> MAPVPEPEVVATPPADAGRGLIRVDSREIRHYSGTRKEPDYLVSRDNGKTWEMKAAPAGYPPNYGGIPKESPAIVRNPLTREFIRVQPIGGFVFLSRGGLDGKWLAVTNDGKLEEDWKDPEKRKNLKKLGGIMRTPVFVNKGRRVIVPFHNMGGGTKFHISDDGGLTWHVSRNGVTSPRHEARPPHQGVRWFNNAVEA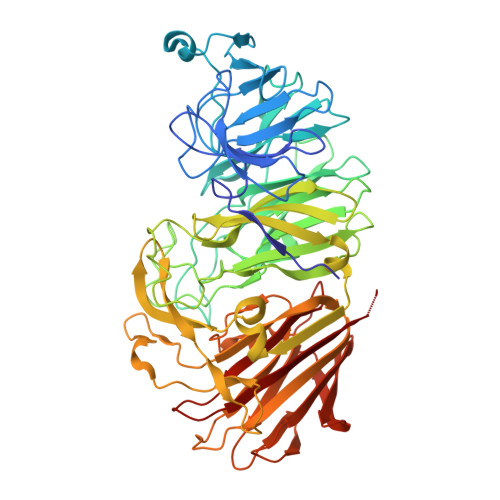TVLEMKDGTLWALARTSQDQAWQAFSKDYGETWSKPEPSRFFGTLTMNTLGRLDDGTIVSLWTNTMALPENATAGNGTWEDVFTNRDSHHIAMSGDEGKTWYGFREIILDEHRNHPGYATLDGPEDRGKHQSEMVQLDKNRILISLGQHKNHRRLVIVDRRWVGAKTRATQTGKDLDSQWTIHTYIPQKKGHCSYNRKPSAELVQDPSGGTKKVLQIKRLDDPELVNEKSNVDYRNGGATWNFPNGTTGLVKFRFRVVDGEQADDSGLQVSLTDRLFNACDSTTKDYALFTFPIRLKPAPHLLLGMKKVPFTPGAWHEISLLWQGGQAVVSLDGKKAGTLKMANKSPNGASYIHFISTGSQPDAGILLDTVNARVKAAAA>MRGSHHHHHHGSMVEKRSVLCFGDSLTWGWIPVKESSPTLRYPYEQRWTGAMAARLGDGYHIIEEGLSARTTSLDDPNDARLNGSTYLPMALASHLPLDLVIIMLGTNDTKSYFHRTPYEIANGMGKLVGQVLTCAGGVGTPYPAPKVLVVAPPPLAPMPDPWFEGMFGGGYEKSKELSGLYKALADFMKVEFFAAGDCISTDGIDGIHLSAETNIRLGHAIADKVAA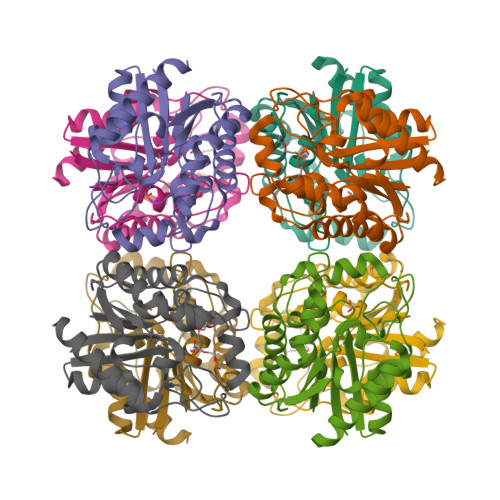LF[4x]>[2x]ADLNTEGDALYSLRQSLKDANNVLQSWDPTLVNPCTWFHVTCNPDNSVIRVDLGNAQLSGALVPQLGQLKNLQYLELYSNNISGTIPNELGNLTNLVSLNLYLNNFTGFIPETLGQLY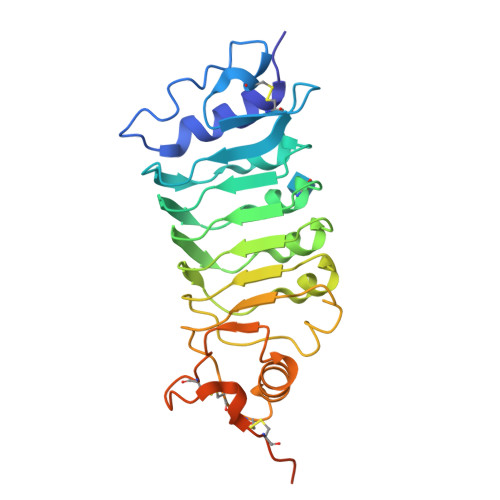KLRFLRLNNNSLSGSIPKSLTNITTLQELALDTNQLKSVPDGIFDRLTSLQKIWLHTNPWDCSCPRIDYLSRWLNKNSQKEQGSAKCSGSGKPVRSIICPTSASLVPRGSWSHPQFEKGSHHHHHH2-[[(2R,3R,4R)-2-(hydroxymethyl)-3-oxidanyl-3,4-dihydro-2H-pyran-4-yl]oxymethyl]-3-methyl-benzimidazole-5-carboxylic acid | C16 H18 N2 O6 | 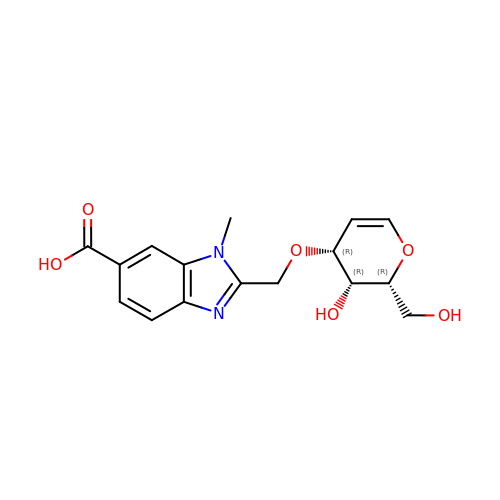QQZYRRIGHJNGGY-UMVBOHGHSA-N>[2x]MGSSHHHHHHSSPRLFMLSSTSSDALRQTARQLATWVEEHQDCVAASDLAYTLARGRAHRPVRTAVVAANLPELVEGLRE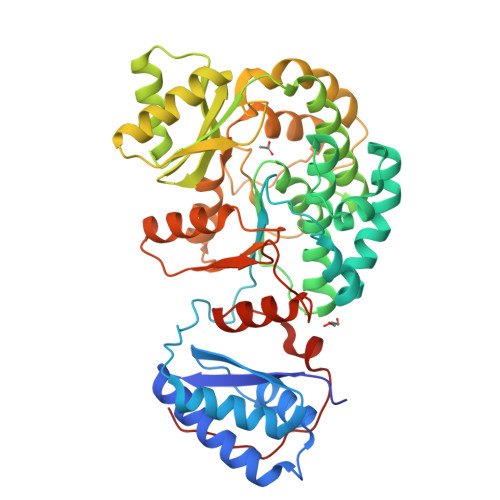VADGDALYDAAVGHGDRGPVWVFSGQGSQWAAMGTQLLASEPVFAATIAKLEPVIAAESGFSVTEAITAQQTVTGIDKVQPAVFAVQVALAATMEQTYGVRPGAVVGHSMGESAAAVVAGALSLEDAARVICRRSKLMTRIAGAGAMGSVELPAKQVNSELMARGIDDVVVSVVASPQSTVIGGTSDTVRDLIARWEQRDVMAREVAVDVAFHSPQVDPILDDLAAALADIAPMTPKVPYYSATLFDPREQPVCDGAYWVDNLRNTVQFAAAVQAAMEDGYRVFAELSPHPLLTHAVEQTGRSLDMSVAALAGMRREQPLPHGLRGLLTELHRAGAALDYSALYPAGRLVDAPLPAWGS>[2x]GSHMLSEELRQIVFRTIESLPEDLRMAITLRELDGLS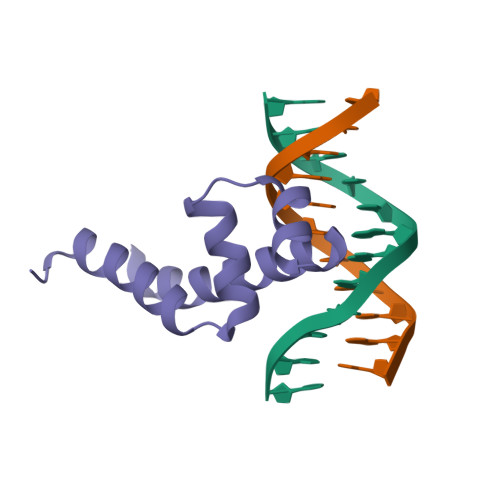YEEIAAIMDCPVGTVRSRIFRAREAIDNKVQPLIRR>[2x]PSVYDAAAQLTADVKKDLRDSW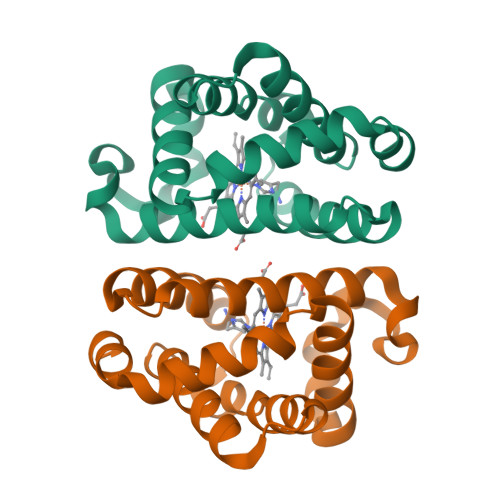KVIGSDKKGNGVAAMTTLFADNQETIGYFKRLGDVSQGMANDKLRGHSITLMYALQNFIDQLDNPDDLVCVVEKFAVNHITRKISAAEFGKINGPIKKVLASKNFGDKYANAWAKLVAVVQAAL>HHHHHHSSGLV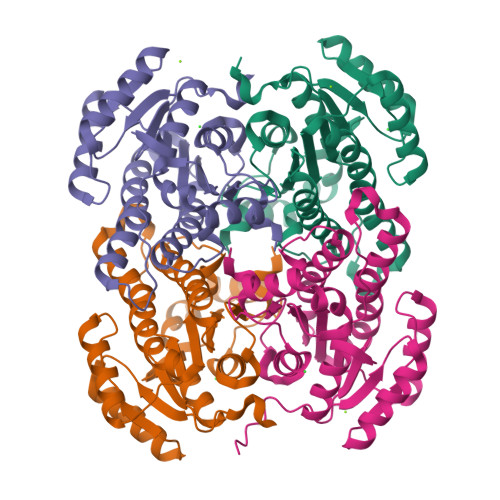PRGSMSNQIIFDLGGRTALVTGSSRGLGRAMAEGLAVAGARILINGTDPSRVAQTVQEFRNVGHDAEAVAFDVTSESEIIEAFARLDEQGIDVDILVNNAGIQFRKPMIELETADWQRVIDTNLTSAFMIGREAAKRMIPRGYGKIVNIGSLTSELARATVAPYTVAKGGIKMLTRAMAAEWAQYGIQANAIGPGYMLTDMNQALIDNPEFDAWVKARTPAKRWGKPQELVGTAVFLSASASDYVNGQIIYVDGGMLSVL[4x]> XTVIN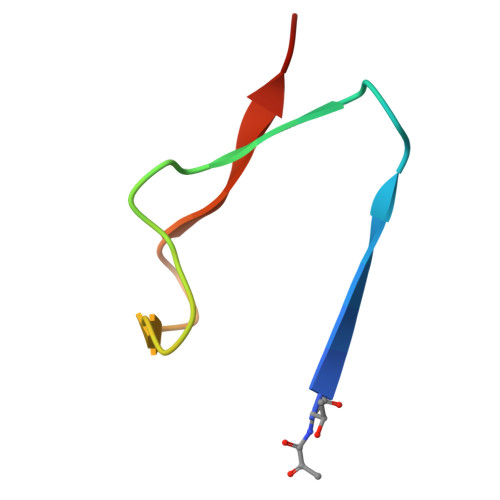LFAPGKVNLVEQLESLSVTKIGQPLAVSTET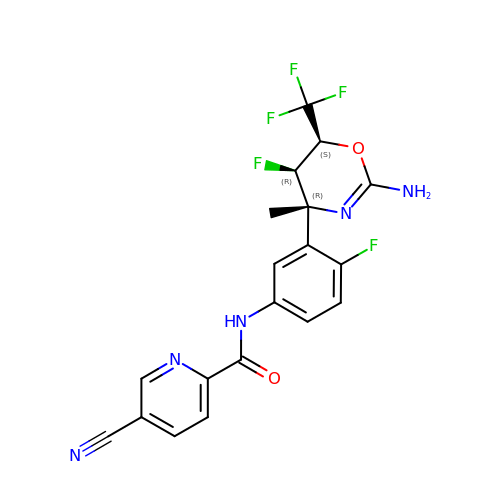N-{3-[(4R,5R,6S)-2-amino-5-fluoro-4-methyl-6-(trifluoromethyl)-5,6-dihydro-4H-1,3-oxazin-4-yl]-4-fluorophenyl}-5-cyanopyridine-2-carboxamide | C19 H14 F5 N5 O2 | UMHIFKHNODSZCU-RLFYNMQTSA-N> GG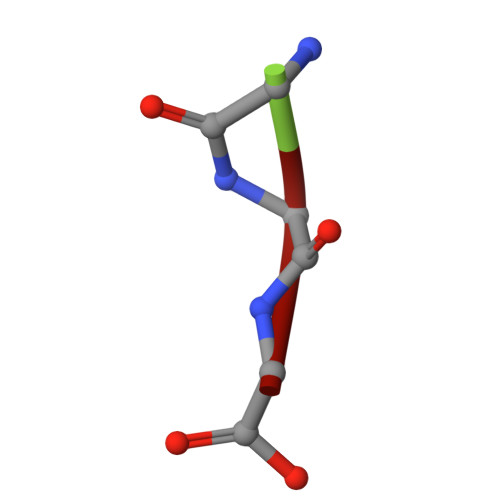G>[3x]GPHMFEARLVQGSILKKVLEALKDLINEACWDISSSGVNLQSMDSSHVSLVQLTLRSEGFDTYRCDRNLAMGVNLTSMSKILKCAGNEDIITLRAEDNADTLALVFEAPNQEKVSDYEMKLMDLDVEQLGIPEQEYSCVVKMPS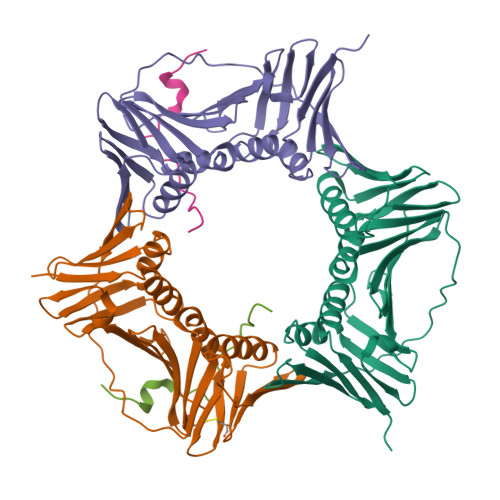GEFARICRDLSHIGDAVVISCAKDGVKFSASGELGNGNIKLSQTSNVDKEEEAVTIEMNEPVQLTFALRYLNFFTKATPLSSTVTLSMSADVPLVVEYKIADMGHLKYYLAPKIEDEEGS;>[2x]APVCVRPTPKWQKGIGEFFAA> MKKFIFATIFALASCAAQPAMAGYDKDLCEWSMTADQTEVETQIEADIMNIVKRDRPEMK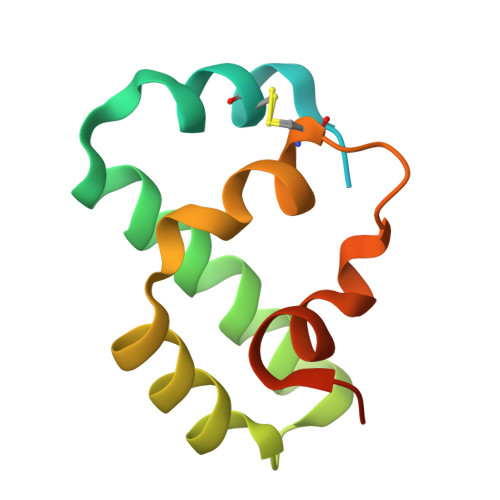AEVQKQLKSGGVMQYNYVLYCDKNFNNKNIIAEVVGELEHHHHHH>[24x]MATEGARNIGQSAPEGKVQMDCPSRHNFDPECEKAFVEHIHLELASSYHAWSMWAFYARDCKAAVGMTRLCEWASHVSAQRARRMAAYVLTRGGHVDYKEIPAPKKQGWDNFEDAFSHCVANKKRILTSLQSLYQCCQSKDAHCSNFIQTDMMDEVIAWNKFLSDCLSNLHCIGSQGMGPWVFDRWLARIVMSKFKHPKIPSLSTSDLESNIPNELFDAEGDMVRAIKKL

The protein artemin acts as both an RNA and protein chaperone and constitutes over 10% of all protein in Artemia cysts during diapause. Artemin monomers are 229 amino-acid residues long with a molecular mass of 26 kDa and form 24mers with a mass of ∼624 kDa. Unlike ferritins whose job is to sequester iron, artemin is unable to bind iron due to naturally modified regions of the ferroxidase center, iron nucleation center and 3-fold channel. Importantly, several biochemical studies point to the chaperone activity of artemin being regulated by a redox switch courtesy of the thiols as well as its C-terminus which diverges considerably from ferritins.

We provide a structure of full-length artemin at 2.04 Å using single particle cryo-EM coupled with cell-free expression. Therefore, octahedral symmetry was imposed in subsequent steps of 3D reconstruction and refinement and led to a final map at 2.04 Å at 0.143 FSC. In total, all residues for artemin except the first 21 N-terminal residues were modeled. Although prior molecular dynamics simulation studies suggested that the C-terminus of artemin forms α-helices that extend inwards into the cavity of the molecule to fill the space, our cryo-EM map of Flag-artemin and the corresponding fitted atomic model clearly show that the C-terminal residues do ultimately turn inwards, but they first hug the inner surface of the core artemin shell before extending only partly into the artemin cavity. Artemin’s loop L′ contains Pro198 and Pro201 which potentially prevents this region from forming into a helical conformation and helps favor the interaction with the inner surface of the shell. A third proline in the C-terminus (Pro213) provides a kink that results in the C-terminal helix F (aa 216–229) turning into the cavity of artemin. In our experimentally derived model, the artemin dimer is oriented similarly to an apoferritin dimer and a disulfide bridge exists between Cys61 and Cys22 of neighboring opposite facing monomers. The overall octahedral symmetry of artemin shows an extra stabilizing interaction relative to apoferritin where the L′ loops or two monomers form a hashtag arrangement that connects the 4-helix bundles from each monomer in addition to the ferritin-like L loop interaction between two monomers at the outer surface. Somewhat surprisingly, loop L′ and helix F extend and contact neighboring dimers which differs from all prior reported homology modeling efforts. This results in helix F from each monomer forming a second 4-helix bundle toward the center of the complex.BIS-1,2-{[(Z)-2CARBOXY-2-METHYL-1,3-DIOXANE]-5-YLOXYCARBONYL}-PIPERAZINE 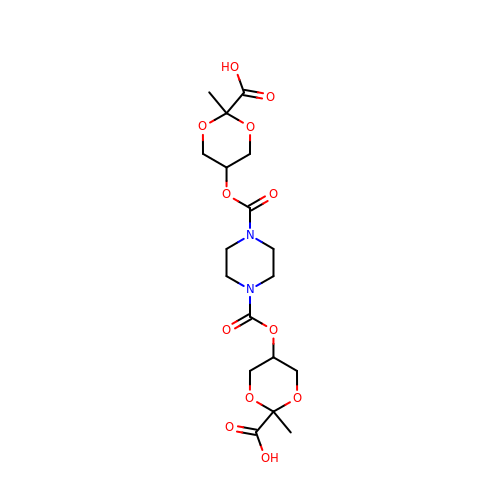| C18 H26 N2 O12 | GNQQJZKGGHOMBD-RDAHUFKRSA-N> KIKACVEEVTTTLEETKFLTENLLLYIDINGNLHPDSATLVSDIDITFLKKDAPYIVGDVVQEGVLTAVVIPTKKAGGTTEMLAKALRKVPTDNYITTYPGQGCNGYTVEEAKTVLKKCKSAFYILPSIISNEKQEILGTVSWNLREMLAHAEETRKLMPVCVETKAIVSTIQRKYKGIKIQEGVVDYGARFYFYTSKTTVASLINTLNDLNETLVTMPLGYVTHGLNLEEAARCMRSLKVPATVSVSSPDAVT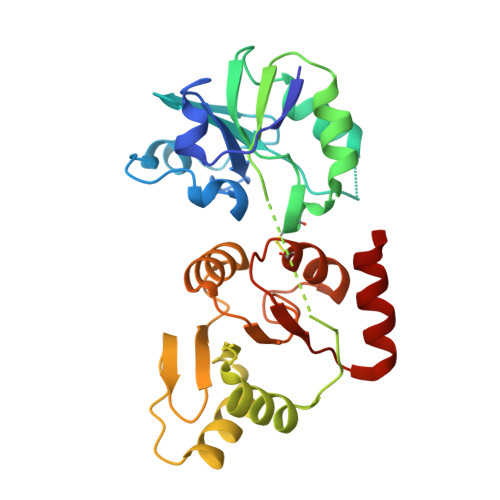AYNGYLTSSS> EHRVLHLRDRLDLAAELKLLCERGPLVRIPLEDGSAVHWFALGYDVVREVLGSEKFDKRVIGTHFNHQEMALPGNLLQLDPPEHTRLRRMVAPAYSVRRMQALEPRVQAIVDDHLDTMASTGPPVEFLREVAGPMAARVACEFLGIPLDDRGELIRLTAHRGGKRRRVLNGHAYLAYMRELAARLRRDPGDGMLGMVARDHGADISDEELAGLCAVVMN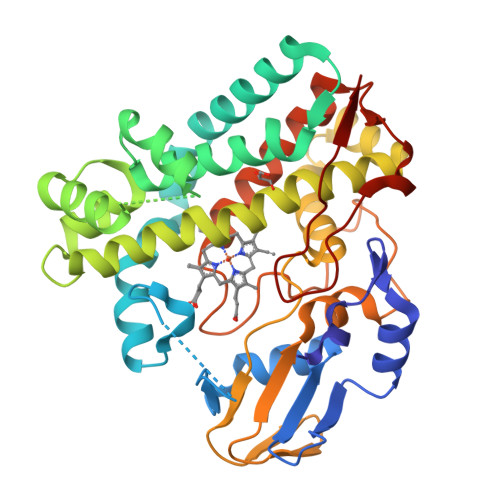SSVEQTESCLAAGTLLLLEHPEQFALLRERPELGEQAVEEIVRYLSVFEGLDPRTATEDVEIGGQVIKKGEAVFCSLLAANRADPALDGFDITRKESRHVAFGHGIHHCLGAPLARMELRIAFTTLVSRFPSLRTAVPAEEIRFRPPSSNVFTLLELPLTW3-O-DECYL-2-DEOXY-6-O-{2-DEOXY-3-O-[(3R)-3-METHOXYDECYL]-6-O-METHYL-2-[(11Z)-OCTADEC-11-ENOYLAMINO]-4-O-PHOSPHONO-BETA-D-GLUCOPYRANOSYL}-2-[(3-OXOTETRADECANOYL)AMINO]-1-O-PHOSPHONO-ALPHA-D-GLUCOPYRANOSE 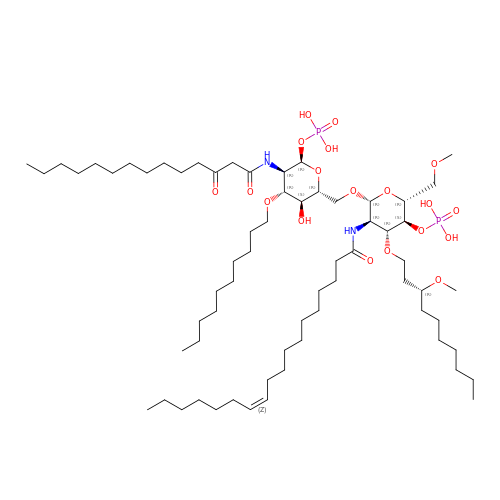| C66 H126 N2 O19 P2 | BPSMYQFMCXXNPC-MFCPCZTFSA-N> GAUAAC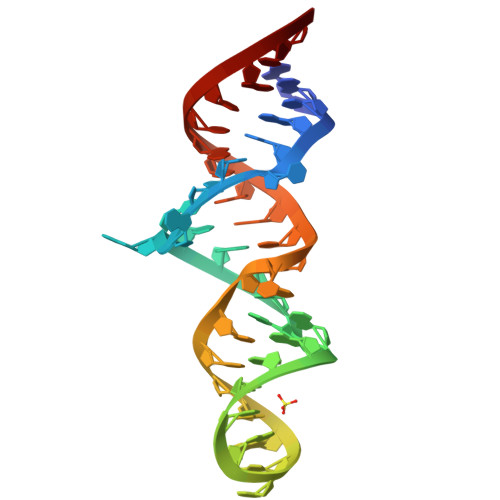UGAAUCGCUAAGGAUGAAAGUCUAUGCGACAUUAUC> MTDQPDLFGLA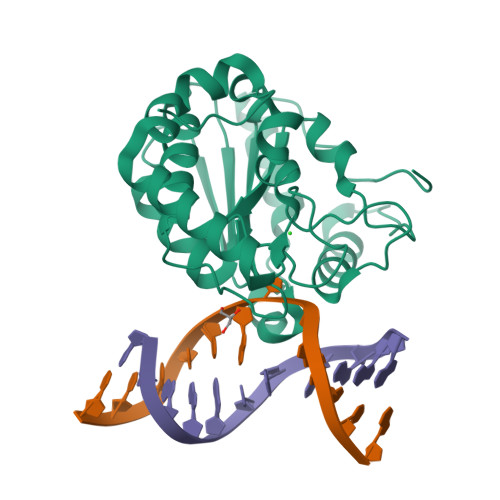PDAPRPIIPANLPEDWQEALLPEFSAPYFHELTDFLRQERKEYTIYPPAPDVFNALRYTPLGEVKVLILGQDPYHGPNQAHGLSFSVRPGVRVPPSLRNIYKELTEDIPGFVAPKHGYLRSWAEQGVLLLNAVLTVRAAQANSHQGKGWEHFTDAVIKAVNAKEERVVFILWGSYARKKKKLITGKNHVVIESGHPSPLSEQYFFGTRPFSKTNEALEKAGRGPVEWQLPATVTEE N-{[(4-aminophenyl)carbonyl]carbamoyl}-beta-D-glucopyranosylamine 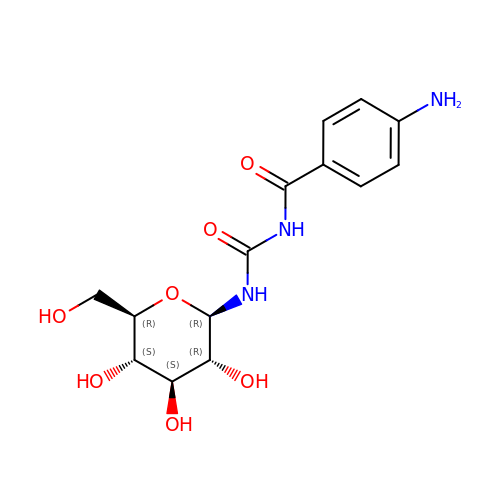| C14 H19 N3 O7 | PVSVRIIRRQSFIR-BZNQNGANSA-N>[2x]UA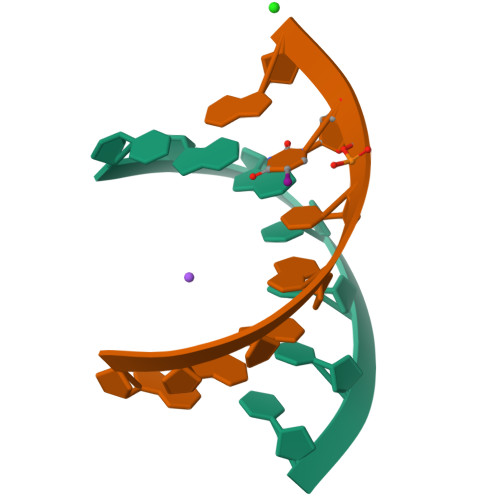GCUCC;>[2x]GGGGCUA>[2x]SAARRALKAVLVDLNGTLHIEDAAVPGAQEALKRLRATSVMVRFVTNTTKETKKDLLERLKKLEFEISEDEIFTSLTAARNLIEQKQVRPMLLLDDRALPEFTGVQTQDPN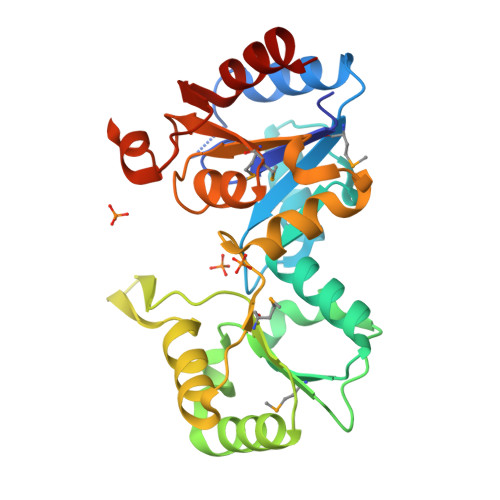AVVIGLAPEHFHYQLLNQAFRLLLDGAPLIAIHKARYYKRKDGLALGPGPFVTALEYATDTKAMVVGKPEKTFFLEALRDADCAPEEAVMIGDDCRDDVDGAQNIGMLGILVKTGKYKAADEEKINPPPYLTCESFPHAVDHILQHLL~{N}-[4-[2,4-bis(fluoranyl)phenoxy]-3-[2-(2-cyclobutyl-1~{H}-imidazol-5-yl)-5-methyl-4-oxidanylidene-furo[3,2-c]pyridin-7-yl]phenyl]ethanesulfonamide 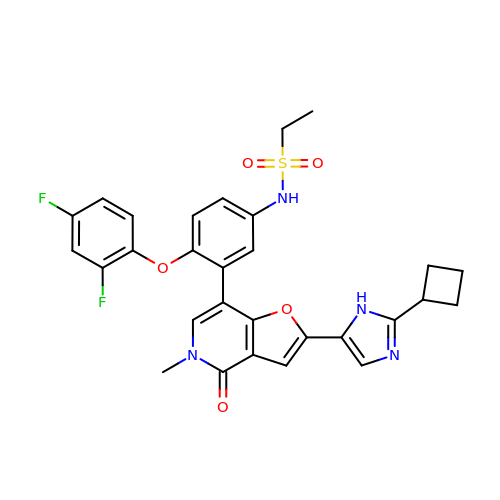| C29 H26 F2 N4 O5 S | JYMKZGYVLHFTMM-UHFFFAOYSA-N>GSKLEFGEIRPTIGQQMETGDQRFGDLVFRQLAPNVWQHTSYLDMPGFGAVASNGLIVRDGGRVLVVDTAWTDDQTAQILNWIKQEINLPVALAVVTHAHQDKMGGMDALHAAGIATYANALSNQLAPQEGMVAAQHSLTFAAN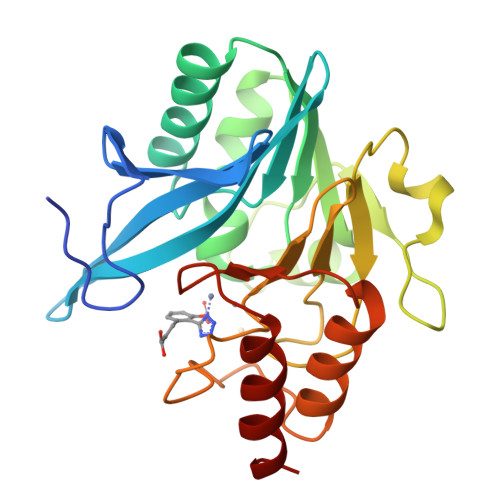GWVEPATAPNFGPLKVFYPGPGHTSDNITVGIDGTDIAFGGCLIKDSKAKSLGNLGDADTEHYAASARAFGAAFPKASMIVMSHSAPDSRAAITHTARMADKLR[2x]>[4x]MKFSNITIKNFRNFEKVNINLDNKNVIFGMNDIGKTNFLYALRFLLDKEIRKFGFNKSDYHKHDTSKKIEIILTLDLSNYEKDEDTKKLISVVKGARTSANADVFYIALESKYDDKELYGNIILKWGSELDNLIDIPGRGNINALDNVFKVIYINPLVDLDKLFAQNKKYIFEESQGNESDEGILNNIKSLTDQVNQQIGEMTIIKGFQQEITSEYRSLKKEEVSIELKSEMAIKGFFSDIIPYIKKDGDSNYYPTSGDGRRKMLSYSIYNYLAKKKYEDKIVIYLIEEPEISLHRSMQIALSKQLFEQSTYKYFFLSTHSPELLYEMDNTRLIRVHSTEKVVCSSHMYNVEEAYGSVKKKLNKALSSALFAERVLLIEGPSEKILFEKVLDEVEPEYELNGGFLLEVGGTYFNHYVCTLNDLGITHIIKTDNDLKSKKGKKGVYELLGLNRCLNLLGRENLDEITIDIPEDIKGKKKKERLNERKKEIFKQYKN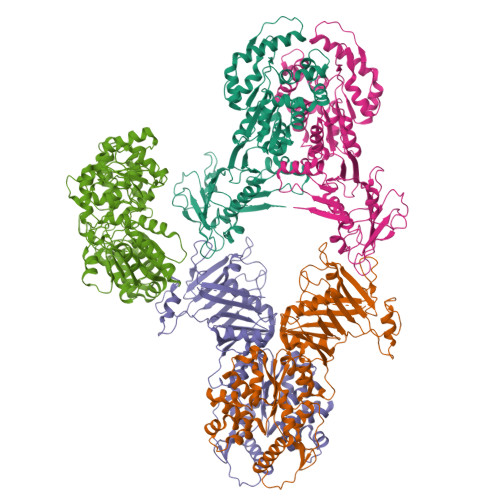EVGEFLGERIYLSEIDLENDLYSAIGESMKRIFENEDPVHYLQKSKLFNMVELVNNLSTKDCFDVFEHEKFACLKELVGSDRG;> MIEDEMSREQIIKDGGNILVTAGAGSGKTTILVSKIEADLKENKTHYSIAAVTFTNKAAKEIEGRLGYSSRGNFIGTNDGFVESEIIRPFIKDAFGNDYPDNFTAEYFDNQFASYDKGLQVLKYQNILGTYSNPKKNFKFQLALDILKKSLVARQYIFSKYFKIFIDEYQDSDKDMHNLFMYLKDQLKIKLFIVGDPKQSIYIWRGAEPENFNGLIENSTDFNKYHLTSNFRCCQDIQNYSNLFNEETRSLIKEKNEVQNVISIADDMPISDILLKLTEEKQVLNIEAELVILVRRRNQAIEIMKELNEEGFNFIFIPQTPLDRATPNATLLKEVIKYVKNDRYSIYDLAAEIVGNLSSREIKEIQKIINELLVPNINQVLINQVLINLFAKLEITLDTREITAFTEVMMTNEFDIAFDTNEYLHKIFTVHSAKGLEFNQVIITASDYNVHYNRDTNEHYVATTRAKDKLIVIMDNKKYSDYIETLMKELKIKNIIKSI>MREVVIVSAVRTAIGSFGGTLKDVSAVDLGAIVIKEAVKRAGIKPEQVDEVIFGNVIQAGVGQSLARQSAVYAGLPVEVPAFTVNKLCGSGLRTVSLAASLISNGDADTIVVGGSENMSASPYLIPKARFGYRMGEAKIYDAMLHDGLIDSFNNYHMGITAENIAEKWGITREDQDKFALASQQKAEAAIKAGKFKDEIVPVTVKMKKKEVVFDTDEDPRFGTTIETLAKLKPAFKRDGTGTVTAGNSSGINDSSAALILMSADKAKELGVKPMAKYVDFASAGLDPAIMGYGPYYATKKVLAKTNLTIKDFDLIEANEAFAAQSIAVARDLEFDMSKVNVNGGAIALGHPVGCSGARILVTLLHEMQKRDAKKGLATLCIGGGQGTAVVVERLEHHHHHH[2x]

Among all r‐BOX or RBO genes, thl_1583, which encodes β‐ketothiolase (MhTHL), is identified as the most critical enzyme for the carbon chain elongation mechanism in M. hexanoica. Therefore, MhTHL is compared with other well‐studied β‐ketothiolases (CkTHL from Clostridium kluyveri, ReBktB from Ralstonia eutropha (Cupriavidus necator), EcAtoB from E. coli, and CaTHL from C. acetobutylicum). In addition, we postulate that the properties of thiolases determine the carbon length of the end products and that the high n‐caproate production of M. hexanoica results from its native thiolase.

The THL from C. kluyveri (CkTHL) was selected as C. kluyveri serves as a model n‐caproate producer. The respective thiolase activities were compared by inserting CkTHL ReBktB, EcAtoB, CaTHL, and MhTHL into the platform strain E. coli SK‐1. The strain containing MhTHL produced more n‐caproate than the strains encoding other thiolase genes, reaching a final concentration of 1.25 g L−1. However, the strain containing CkTHL produced a similar level (≈0.9 g L−1) of n‐caproate as MhTHL. We then superimposed the MhTHL structure on the crystal structures of well‐known thiolases, such as EcAtoB, ReBktB, CaTHL, and CkTHL, to investigate their structural differences. The overall structures were relatively identical, with alpha carbon RMS distances of 0.50, 0.62, 0.53, and 0.46, respectively. L87 and V351 in MhTHL and the corresponding L87 and V352 in CkTHL modulated the pocket size to a greater extent than the valine and isoleucine residues in EcAtoB and CaTHL. In the case of ReBktB, the protein contains Leu89 and Ile352 at the positions, making the pocket larger than CaTHL but smaller than CkTHL and MhTHL. This corresponds to the n‐caproate production results in the platform strain SK‐1 with altered thiolases.>[4x]MNEQAILQSAEAWVKKQLMDEYSGHDWYHIRRVTLMAKAIGEQEKVDVFVVQIAALFHDLIDDKLVDDPETAKQQLIDWMEAAGVPSQKIDHTMDIINTISFKGGHGQSLATREAMVVQD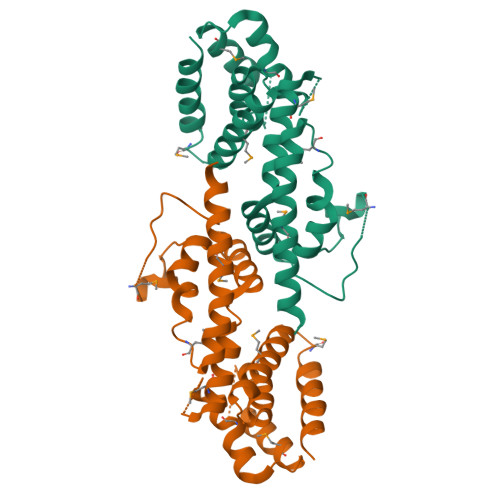ADRLDALGAIGIARTFAYSGNKGQPIYDPELPIRETMTVEEYRHGKSTAINHFYEKLFKLKDLMNTETGKQLAKERHVFMEQFIERFLSEWNGDMLEHHHHHH> MLLGSSEESQAFQRQLTALIGYDVTDVSNVHDDELEFTRRGLVTPRMAEVASRDPKLYAMHPWVTSKPLPEYLWKKIANNCIFIVIHR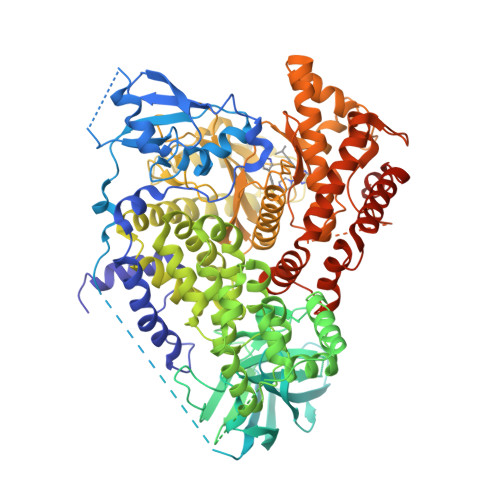STTSQTIKVSPDDTPGAILQSFFTKMAKKKSLMDIPESQSEQDFVLRVCGRDEYLVGETPIKNFQWVRHCLKNGEEIHVVLDTPPDPALDEVRKEEWPLVDDCTGVTGYHEQLTIHGKDHESVFTVSLWDCDRKFRVKIRGIDIPVLPRNTDLTVFVEANIQHGQQVLCQRRTSPKPFTEEVLWNVWLEFSIKIKDLPKGALLNLQIYCGKAPALSSKASAESPSSESKGKVQLLYYVNLLLIDHRFLLRRGEYVLHMWQISGKGEDQGSFNADKLTSATNPDKENSMSISILLDNYCHPIALPKHQPTPDPEGDRVRAEMPNQLRKQLEAIIATDPLNPLTAEDKELLWHFRYESLKHPKAYPKLFSSVKWGQQEIVAKTYQLLARREVWDQSALDVGLTMQLLDCNFSDENVRAIAVQKLESLEDDDVLHYLLQLVQAVKFEPYHDSALARFLLKRGLRNKRIGHFLFWFLRSEIAQSRHYQQRFAVILEAYLRGCGTAMLHDFTQQVQVIEMLQKVTLDIKSLSAEKYDVSSQVISQLKQKLENLQNSQLPESFRVPYDPGLKAGALAIEKCKVMASKKKPLWLEFKCADPTALSNETIGIIFKHGDDLRQDMLILQILRIMESIWETESLDLCLLPYGCISTGDKIGMIEIVKDATTIAKIQQSTVGNTGAFKDEVLNHWLKEKSPTEEKFQAAVERFVYSCAGYCVATFVLGIGDRHNDNIMITETGNLFHIDFGHINGNYKSFLGINKERVPFVLTPDFLFVMGTSGKKTSPHFQKFQDICVKAYLALRHHTNLLIILFSMMLMTGMPQLTSKEDIEYIRDALTVGKNEEDAKKYFLDQIEVCRDKGWTVQFNWFLHLVLGIKQGEKHSAEFGLVPRGSGHHHHHH> GIGTGFPFDPHYVEVLGERMHYVDVGPRDGTPVLFLHGNPTSSYVWRNIIPHVAPTHRCIAPDLIGMGKSDKPDLGYFFDDHVRFMDAFIEALGLEEVVLVIHDWGSALGFHWAKRNPERVKGIAFMEFIRPIPTWDEWPKFARKTFQAFRTKKVGRKLIIDQNVFIEGTLPMGVVRPLTEVEMDHYREPFLNPVDREPLWRFPNELPIAGEPANIVALVEEYMDWLHQSPVPKLLFWGTPGVLIPPAEAARLAKSLPNCKAVDIGPGLNLLQEDNPDLIGSE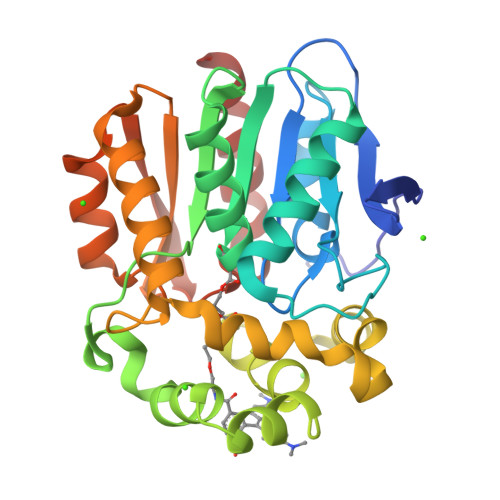IARWLSTLEISG> YEQDKTYKITVLHTNDHHGHFWRNEYGEYGLAAQKTLVDGIRKEVAAEGGSVLLLSGGDINTGVPESDLQDAEPDFRGMNLVGYDAMAIGNHEFDNPLTVLRQQEKWAKFPLLSANIYQKSTGERLFKPWALFKRQDLKIAVIGLTTDDTAK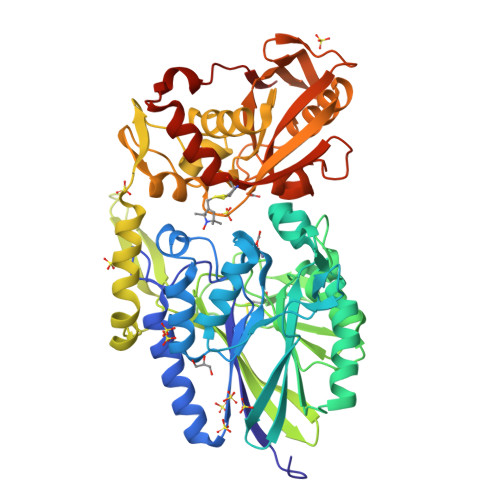IGNPEYFTDIEFRKPADEAKLVIQELQQTEKPDIIIAATHMGHYDNGEHGSNAPGDVEMARALPAGSLAMIVGGHSQDPVCMAAENKKQVDYVPGTPCKPDQQNGIWIVQAHEWGKYVGRADFEFRNGEMKMVNYQLIPVNLKKKVTWEDGKSERVLYTPEIAENQQMISLLSPFQNKGKAQLEVKIGETNGRLEGDRDKVRFVQTNMGRLILAAQMDRTGADFAVMSGGGIRDSIEAGDISYKNVLKVQPFGNVVVYADMTGKEVIDYLTAVAQMKPDSGAYPQFANVSFVAKDGKLNDLKIKGEPVDPAKTYRMATLNFNATGGDGYPRLDNKPGYVNTGFCDAEVLKAYIQKSSPLDVSVYEPKGEVSWQLEHHHHHH> MVDDAGAAESQRGKQTPAHSLEQLRRLPLPPPQIRIRPWWFPVQELRDPLVFYLEAWLADELFGPDRAIIPEMEWTSQ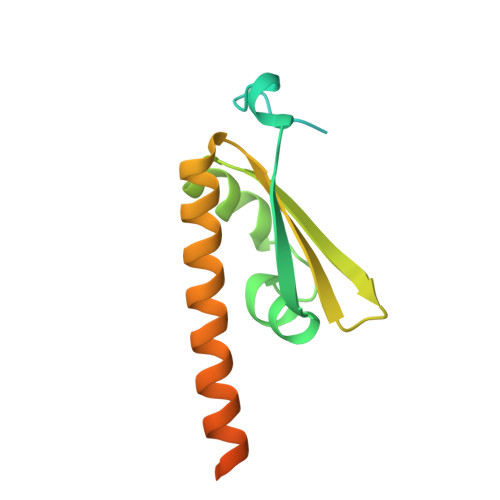ALLTVDIVDSGNLVEITVFGRPRVQNRVKSMLLCLAWFHREHRARAEKMKHLEKNLKAHASDPHSPQDPVA(2~{R},4~{S})-5,5-dimethyl-2-[(2~{S},3~{R})-3-oxidanyl-1-oxidanylidene-5-thiophen-2-yl-pentan-2-yl]-1,3-thiazolidine-4-carboxylic 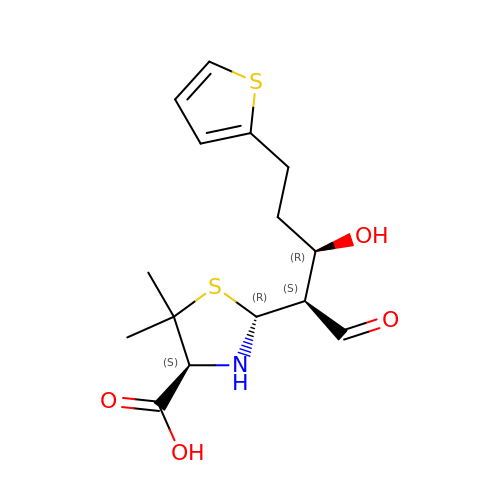acid | C15 H21 N O4 S2 | RTEPAFLPRWPVOF-FVCCEPFGSA-N> QRAEEEDD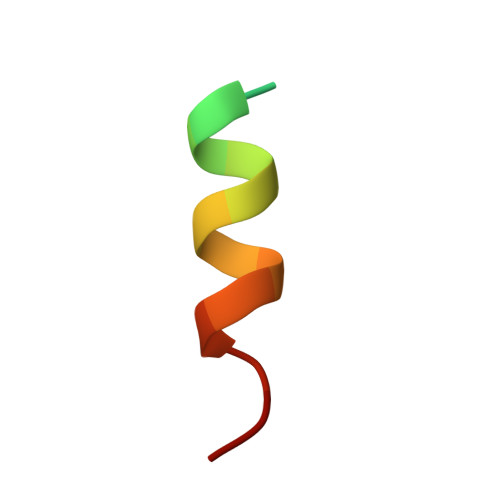DIKQLAAWTT>[4x]MAHHHHHHSSGLEVLFQGPMSSNMIKADCVVIEDSFRGFPTEYFCTSPRYDECLDYV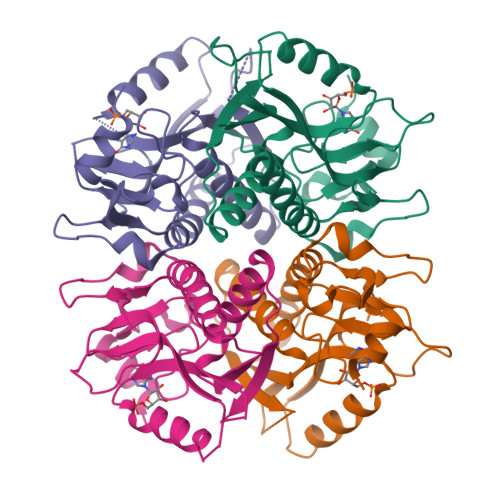LIPNGMIKDRLEKMSMNIVDYYEACNATSITLMCVLKGGFKFLADLVDGLERTVRARGIVLPMSVEFVRVKSYVNDVSIHEPILTGLGDPSEYKDKNVLVVEDIIDTGKTITKLISHLDSLSTKSVKVASLLVKRTSPRNDYRPDFVGFEVPNRFVVGYALDYNDNFRDLHHICVINEVGQKKFSVPCTSKPV> QDNLYEEIQKHAKQYEIAPQNAMIDKIWKATPGYNGRQVDMEASYNNMKKLKKFDQKHLEFKEVSPSVHLEDLSPAPIYRGHPNKKMVGLTIDVAWGNEYLPRILEILKKHDVKATFFLEGRWVKENLRFAKMIVDANQEVGNHSYTHPNMKTLSSDEIRDQLQKTNRMIEAATNQKVRWFAPPSGSFRDEVVK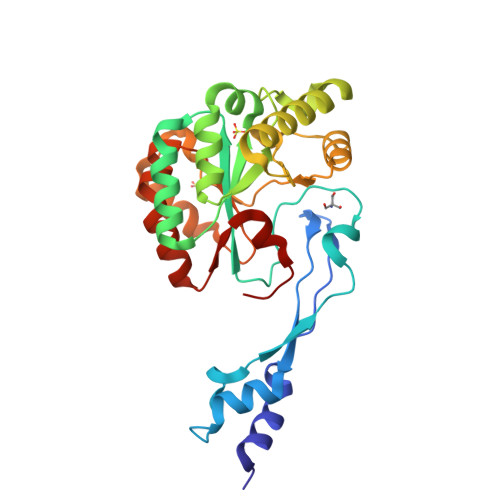IADDFQMGTIMWTVDTIDWKRPEPDVLLQRVMRKIHPGAIVLMHPTSSTTEALDTMITKLKEQGYKVGNITELLDEKRV>[2x]MTGPILSGLDPRFERTLYAHVGKEGSWTLDYYLRHGGYETAKRVLKEKTPDEVIEEVKRSGLRGRGGAGFPTGLKWSFMPKDDGKQHYLICNADESEPGSFKDRYILEDVPHLLIEGMILAGYAIRATVGYIYVRGEYRRAADRLEQAIKEARARGYLGKNLFGTDFSFDLHVHRGAGAYICGEETALMNSLEGLRANPRLKPPFPAQSGLWGKPTTINNVETLASVVPIMERGADWFAQMGTEQSKGMKLYQISGPVKRPGVYELPMGTTFRELIYEWAGGPLEPIQAIIPGGSSTPPLPFTEEVLDTPMSYEHLQAKGSMLGTGGVILIPERVSMVDAMWNLTRFYAHESCGKCTPCREGVAGFMVNLFAKIGTGQGEEKDVENLEALLPLIEGRSFCPLADAAVWPVKGSLRHFKDQYLALAREKRPVPRPSLWR;>[2x]MGFFDDKQDFLEETFAKYPPEGRRAAIMPLLRRVQQEEGWIRPERIEEIARLVGTTPTEVMGVASFYSYYQFVPTGKYHLQVCATLSCKLAGAEELWDYLTETLGIGPGEVTPDGLFSVQKVECLGSCHTAPVIQVNDEPYVECVTRARLEALLAGLRAGKRLEEIELPGKCGHHVHEVEV;>MVRVKVNDRIVEVPPGTSVMDAVFHAGYDVPLFCSEKHLSPIGACRMCLVRIGLPKKGPDGKPLLNEKGEPEIQWQPKLAASCVTAVADGMVVDTLSDVVREAQAGMVEFTLLNHPLDCPTCDKGGACELQDRTVEYGLYEKYYQKGPLELPVYTRFEFTRRHVDKHHPLSPFVILDRERCIHCKRCVRYFEEVPGDEVLDFIERGVHTFIGTMDFGLPSGFSGNITDICPVGALLDLTARFRARNWEMEETPTTCAL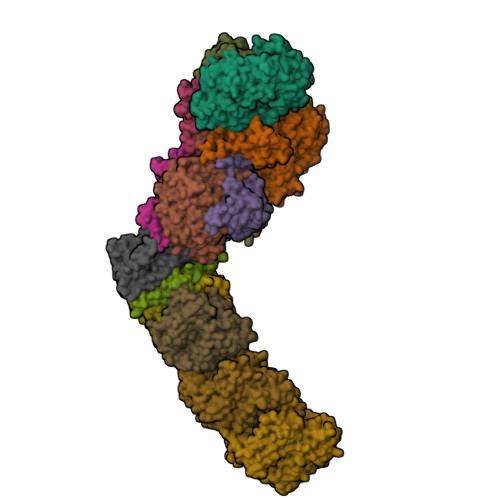CPVGCGITADTRSGELLRIRAREVPEVNEIWICDAGRFGHEWADQNRLKTPLVRKEGRLVEATWEEAFLALKEGLKEARGEEVGLYLAHDATLEEGLLASELAKALKTPHLDFQGRTAAPASLFPPASLEDLLQADFALVLGDPTEEAPILHLRLSEFVRDLKPPHRYNHGTPFADLQIKERMPRRTDKMALFAPYRAPLMKWAAIHEVHRPGEEREILLALLGDKEGSEMVAKAKEAWEKAKNPVLILGAGVLQDTVAAERARLLAERKGAKVLAMTPAANARGLEAMGVLPGAKGASWDEPGALYAYYGFVPPEEALKGKRFVVMHLSHLHPLAERYAHVVLPAPTFYEKRGHLVNLEGRVLPLSPAPIENGEAEGALQVLALLAEALGVRPPFRLHLEAQKALKARKVPEAMGRLSFRLKELRPKERKGAFYLRPTMWKAHQAVGKAQEAARAELWAHPETARAEALPEGAQVAVETPFGRVEARVVHREDVPKGHLYLSALGPAAGLRVEGRVLVPAGGEA[2x];>MREEFLEEIPLDAPPEEAKELRTEVMTLNVGPQHPSTHGVLRLMVTLSGEEVLEVVPHIGYLHTGFEKTMEHRTYLQNITYTPRMDYLHSFAHDLAYALAVEKLLGAVVPPRAETIRVILNELSRLASHLVFLGTGLLDLGALTPFFYAFRERETILDLFEWVTGQRFHHNYIRIGGVKEDLPEEFVPELKKLLEVLPHRIDEYEALFAESPIFYERARGVGVIPPEVAIDLGLTGGSLRASGVNYDVRKAYPYSGYETYTFDVPLGERGDVFDRMLVRIREMRESVKIIKQALERLEPGPVRDPNPQITPPPRHLLETSMEAVIYHFKHYTEGFHPPKGEVYVPTESARGELGYYIVSDGGSMPYRVKVRAPSFVNLQSLPYACKGEQVPDMVAIIASLDPVMGDVDR[2x];>[2x]MRLERVLEEARAKGYPIEDNGLGNLWVVLPRERFKEEMAHYKAMGFNFLADIVGLDYLTYPDPRPERFAVVYELVSLPGWKDGDGSRFFVRVYVPEEDPRLPTVTDLWGSANFLEREVYDLFGIVFEGHPDLRKILTPEDLEGHPLRKDYPLGETPTLFREGRYIIPAEFRAALTGKDPGLTFYKGGSRKGYRSLWADLKKAREVKG;>[2x]MALKDLFERDVQELEREGILFTTLEKLVAWGRSNSLWPATFGLACCAIEMMASTDARNDLARFGSEVFRASPRQADVMIVAGRLSKKMAPVMRRVWEQMPDPKWVISMGACASSGGMFNNYAIVQNVDSVVPVDVYVPGCPPRPEALIYAVMQLQKKVRGQAYNERGERLPPVAAWKRTRG;>[2x]MSASSERELYEAWVELLSWMREYAQAKGVRFEKEADFPDFIYRMERPYDLPTTIMTASLSDGLGEPFLLADVSPRHAKLKRIGLRLPRAHIHLHAHYEPGKGLVTGKIPLTKERFFALADRAREALAFA;>MTLKALAQSLGITLKYLFSKPVTVPYPDAPVALKPRFHGRHVLTRHPNGLEKCIGCSLCAAACPAYAIYVEPAENDPENPVSAGERYAKVYEINMLRCIFCGLCEEACPTGAIVLGYDFEMADYEYSDLVYGKEDMLVDVVGTKPQRREAKRTGKPVKVGYVVPYVRPELEGFKAPTEGGKR[2x];>MAPIQEYVGTLIYVGVALFIGVAALLVGALLGPKKPGRAKLMPYESGNDPAGEVKRFPVHFYVVAMLFILFDVEVAFLWPYAVSAGGLGLYGFLGVLAFTLLLFVGFLYEWWKGVMRWH[2x];>MTWSYPVDPYWMVALKALLVVVGLLTAFAFMTLIERRLLARFQVRMGPNRVGPFGLLQPLADAIKSIFKEDIVVAQADRFLFVLAPLISVVFALLAFGLIPFGPPGSFFGYQPWVINLDLGILYLFAVSELAVYGIFLSGWASGSKYSLLGSLRSSASLISYELGLGLALLAPVLLVGSLNLNDIVNWQKEHGWLFLYAFPAFLVYLIASMAEAARTPFDLPEAEQELVGGYHTEYSSIKWALFQMAEYIHFITASALIPTLFLGGWTMPVLEVPYLWMFLKIAFFLFFFIWIRATWFRLRYDQLLRFGWGFLFPLALLWFLVTALVVALDLPRTYLLYLSALSFLVLLGAVLYTPKPARKGGGA[2x];>MSLLEGLALFLLLLSGVLVVTLRNAIHAALALILNFLVLAGVYVALDARFLGFIQVIVYAGAIVVLFLFVIMLLFAAQGEIGFDPLVRSRPLAALLALGVAGILAAGLWGLDLAFTQDLKGGLPQALGPLLYGDWLFVLLAVGFLLMAATVVAVALVEPGKASRAKEAEKREEVAR[2x];>[2x]MSYLLTSALLFALGVYGVLTRRTAILVFLSIELMLNAANLSLVGFARAYGLDGQVAALMVIAVAAAEVAVGLGLIVAIFRHRESTAVDDLSELRG;>[2x]MALLGTILLPLLGFALLGLFGKRMREPLPGVLASGLVLASFLLGAGLLLSGGARFQAEWLPGIPFSLLLDNLSGFMLLIVTGVGFLIHVYAIGYMGGDPGYSRFFAYFNLFIAMMLTLVLADSYPVMFIGWEGVGLASFLLIGFWYKNPQYADSARKAFIVNRIGDLGFMLGMAILWALYGTLSISELKEAMEGPLKNPDLLALAGLLLFLGAVGKSAQIPLMVWLPDAMAGPTPVSALIHAATMVTAGVYLIARSSFLYSVLPDVSYAIAVVGLLTAAYGALSAFGQTDIKKIVAYSTISQLGYMFLAAGVGAYWVALFHVFTHAFFKALLFLASGSVIHALGGEQDVRKMGGLWKHLPQTRWHALIGALALGGLPLLSGFWSKDAILAATLTYPFGGVGFYVGALLVAVLTAMYAMRWFVLVFLGEERGHHHPHEAPPVMLWPNHLLALGSVLAGYLALPHPLPNVLEPFLKPALAEVEAHHLSLGAEWGLIALSAAVALLGLWAGFVFFQRKVFPAWYLAFEAASREAFYVDRAYNALIVNPLKALAEALFYGDRGLLSGYFGLGGAARSLGQGLARLQTGYLRVYALLFVLGALLLLGVMRW;>[2x]MVVLAVLLPVVFGALLLLGLPRALGVLGAGLSFLLNLYLFLTHPGGVAHAFQAPLLPGAGVYWAFGLDGLSALFFLTIALTVFLGALVARVEGRFLGLALLMEGLLLGLFAARDLLVFYVFFEAALIPALLMLYLYGGEGRTRALYTFVLFTLVGSLPMLAAVLGARLLSGSPTFLLEDLLAHPLQEEAAFWVFLGFALAFAIKTPLFPLHAWLPPFHQENHPSGLADALGTLYKVGVFAFFRFAIPLAPEGFAQAQGLLLFLAALSALYGAWVAFAAKDFKTLLAYAGLSHMGVAALGVFSGTPEGAMGGLYLLAASGVYTGGLFLLAGRLYERTGTLEIGRYRGLAQSAPGLAALALILFLAMVGLPGLSGFPGEFLTLLGAYKASPWLAALAFLSVIASAAYALTAFQKTFWEEGGSGVKDLAGAEWGFALLSVLALLLMGVFPGYFARGLHPLAEAFAKLLGGGA;>MTLAILAVFSVALTLLGFVLPPQGVKRATLLGLALALASLLLTWGKPFAFGPYAVDGVSQVFTLLALLGALWTVGLVRSGRFEFYLLVLYAALGMHLLASTRHLLLMLVALEALSLPLYALATWRRGQGLEAALKYFLLGALAAAFFLYGAALFYGATGSLVLGAPGEGPLYALALGLLLVGLGFKAALAPFHFWTPDVYQGSPTPVVLFMATSVKAAAFAALLRVAAPPEALALLVALSVVVGNLAALAQKEAKRLLAYSSIAHAGYMALALYTGNAQALGFYLLTYVLATGLAFAVLSQISPDRVPLEALRGLYRKDPLLGLAFLVAMLSLLGLPPLAGFWGKYLAFAEAARAGAWGVLVLALVTSAVSAYYYLGLGLAVFARPEETPFRPGPPWARAAVVAAGVLLLALGLLPGLVLPALAAGG[2x];>[2x]MVRVGMRAAPRVSLEALKAALGGLKLSEAKVYLITDWQDKRDQARYALLLHTGKKDLLVPDAFGPAFPGGEEALSELVGLLLAQGARRFYEAVVSPGEMTALLDLPPEELLKRVMAIANPTDPGIYLKRAA> MKTEWPELVG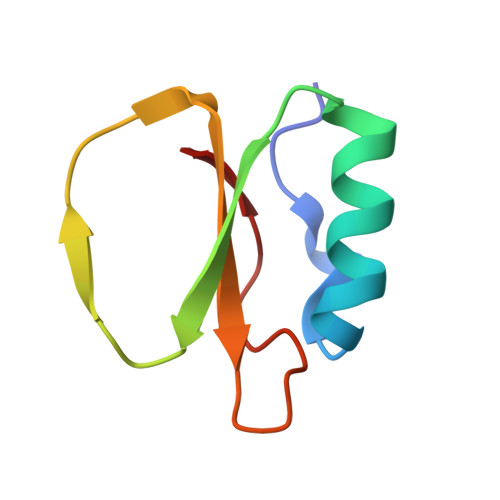KSVEEAKKVILQDKPAAQIIVLPVGTIVTGEYRIDRVRLFVDRLDNIAQVPRVG>SQGHKPLEVIKIEDGVYLHTSFKNIEGYGLVDSNGLVVLDNNQAYIIDTPWSEEDTKLLLSWATDRGYQVMASISTHSHEDRTAGIKLLN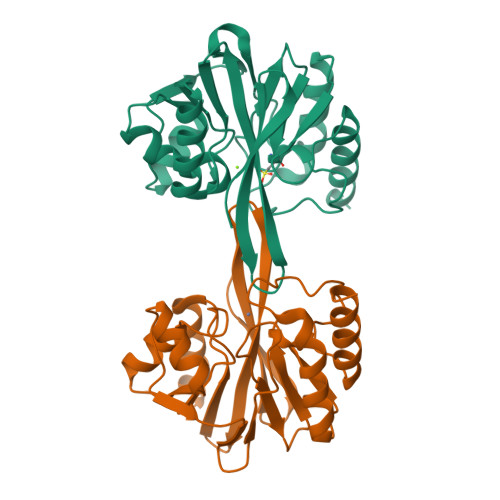SKSIPTYTSELTKKLLAREGKPVPTHYFKDDEFTLGNGLIELYYPGAGHTEDNIVAWLPKSKILFGGCLVRSHEWEGLGYVGDASISSWADSIKNIVSKKYPIQMVVPGHGKVGSSDILDHTIDLAESASNKLMQPTAEASAD[2x]> MEANGLGPQGFPELKNDTFLRAAWGEETDYTPVWCMRQAGRYLPEFRETRAAQDFFSTCRSPEACCELTLQPLRRFPLDAAIIFSDILVVPQALGMEVTMVPGKGPSFPEPLREEQDLERLRDPEVVASELGYVFQAITLTRQRLAGRVPLIGFAGAPWTLMTYMVEGGGSSTMAQAKRWLYQRPQASHQLLRILTDALVPYLVGQVVAGAQALQLFESHAGHLGPQLFNKFALPYIRDVAKQVKARLREAGLAPVPMIIFAKDGHFALEELAQAGYEVVG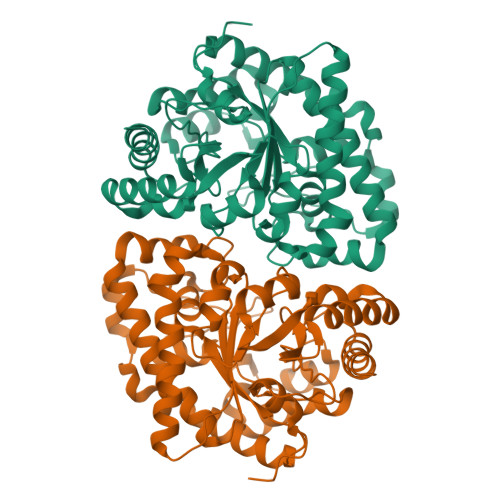LDWTVAPKKARECVGKTVTLQGNLDPCALYASEEEIGQLVKQMLDDFGPHRYIANLGHGLYPDMDPEHVGAFVDAVHKHSRLLRQN>MKFYTISSKYIEYLKEFDDKVPNSEDPTYQNPKAFIGIVLEIQGHKYLAPLTSPKKWHNNVKESSLSCFKLHENGVPENQLGLINLKFMIPIIEAEVSLLDLGNMPNTPYKRMLYKQLQFIRANSDKIASKSDTLRNLVLQGKMQGTCNFSLLEEKYRD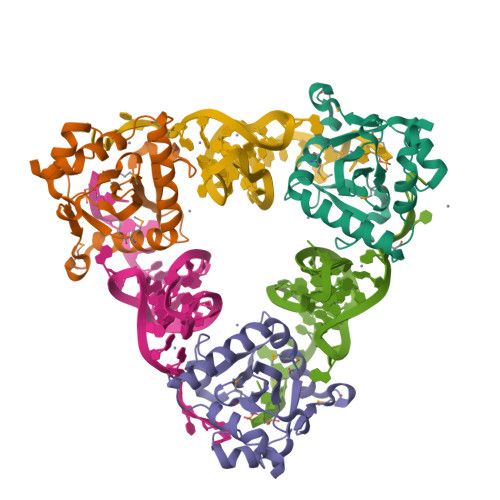FGKEAEDTEEGE[3x]2-amino-8-sulfanyl-1,9-dihydro-6H-purin-6-one 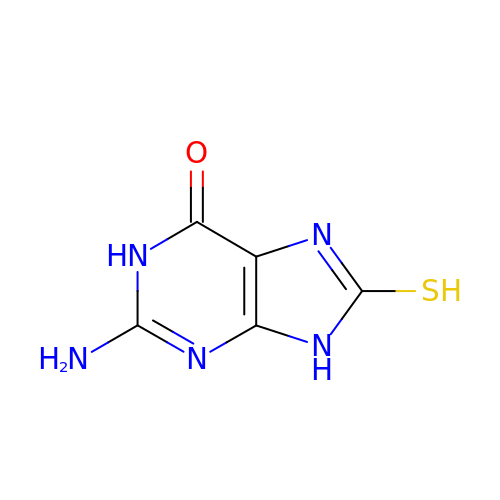| C5 H5 N5 O S | JHEKNTQSGTVPAO-UHFFFAOYSA-N>[2x]DVQEQDIETLHGSVHVTLCGTPKGNRPVILTYHDIGMNHKTCYNPLFNYEDMQEITQHFAVCHVDAPGQQDGAASFPAGYMYPSMDQLAEMLPGVLQQFGLKSIIGMGTGAGAYILTRFALNNPEMVE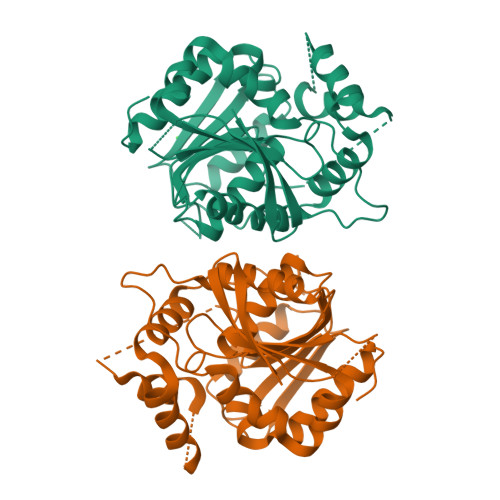GLVLINVNPCAEGWMDWAASKISGWTQALPDMVVSHLFGKEEMQSNVEVVHTYRQHIVNDMNPGNLHLFINAYNSRRDLEIERPMPGTHTVTLQCPALLVVGDSSPAVDAVVECNSKLDPTKTTLLKMADCGGLPQISQPAKLAEAFKYFVQGMGYMPSAS>[3x]MSVYFFD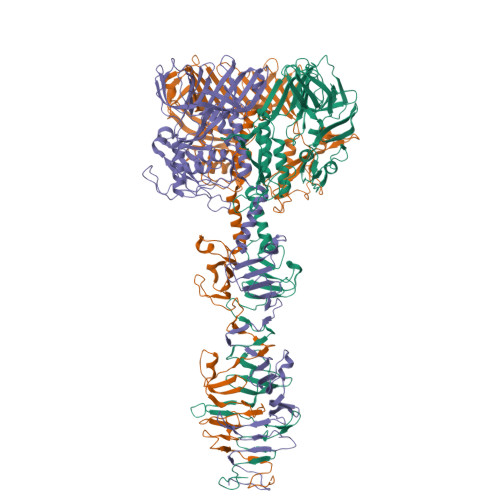NKQQLIKIKNSRTLLQCLQEKEIASDKSDLMKDVLTVSCLHDVELEQCDFMAVRENKGVYSLYKILEEEIDAEIMNFKGVNFGAEELNNYVVSDARPVKKTITEIVKQILTYTDDEWLMTGGVNKIGSANFYYASVKEALKTVQQLGCELLFFCDIDGEGISSKWVEVREKIGKESDDRYEVGSTAIKVVKTKDRTNIVTSLVGRGKGEEVGDGYGRRLQFDSIEWTQPVPKPKGQSFIEIKELTEKYGIPTKKGKMRKREQVVIFEDIEDKNELLNATYQTLLENSRPLVQFSSEVIGASSIGDMVTIHDYDKNYHYETRVFAIKNDILNNKIESSLGDNLKGSSASNQLSKASSGISELKSMKMNFYDSTEISKWQSDIIRGAKGGSVLLMSPWDTNKGQSREPYQMVIMNKGSLKESNHFLVMNSEGIGFIDGDFDKDKFETAWTIDGTFNAKFIRAGVLSGILIKGNIIKSSDEGDFQIVLDGGELTFEKKYDSEDINDQHGHPMLTMKALYTDDKLNGISMVQIPNYSFGINSGGLMVSKPVIEIPKESTIDSRKLNLFGEVRVVGDFYVNDVKIDSNGGSGGSGGGSGGWNGQYPPEITSDVDKRAWAIWSTSRGLGYSKAAAAAKLGNIQGESGPQMNPDTEQVGGPAYGLVQWDGSAYPLVGQPTNNGREYVQRLMKAANITDDYRTIVPQVNLIEWSMKNGQWIGAVEPKTVSGFKASISPRTAARAFLYNFERPATGHPEREDYAQAWYDKFKDLKQPGGKYGMPVGPGYQITSWFGNRDNPTDPGNIETHKGMDFADKIGSPIFAVEKGEVFASLSTGSSGGFGEYIVIKHEDGNFTGYAHMTLRMLETGAKVSKGQQIGTLGSTGESTGPHLHFSVGDGLFGNYQDPAPYLGLKRP N-ethyl-N-({3-[1-(4-methylphenyl)cyclopentyl]-1,2,4-oxadiazol-5-yl}methyl)-2-(1H-pyrazol-1-yl)ethan-1-amine | C22 H29 N5 O | 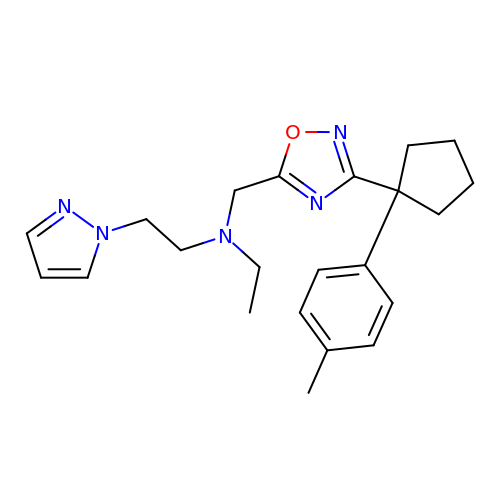CIGIIVQVOWUOHH-UHFFFAOYSA-N>GGNAAEVNLDELAQELGPIMGDNEQLALAYRVIRDMFVFTNKRLILIDKQGVTGKKVSYHSVPYKAITHFEVETAGTFDMDAELKLWISGQKDPLVKELKKGTDVVGI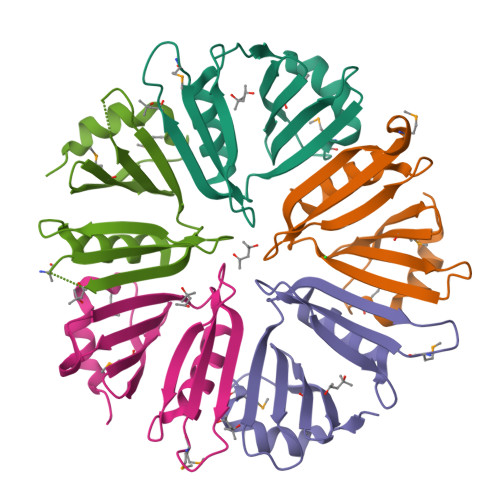QKTIANFSL[5x]(1R)-1-(naphthalen-2-yl)ethane-1,2-diol | C12 H12 O2 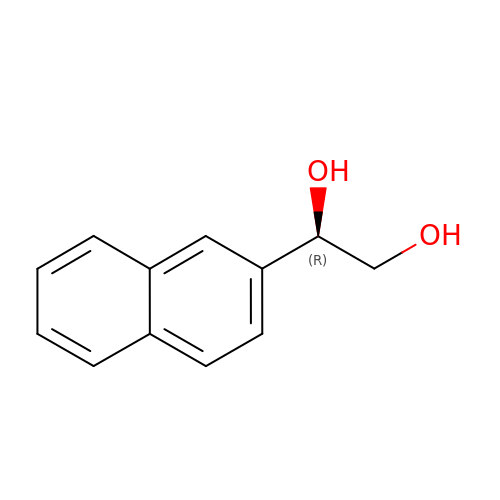| QFNOPZNUHSDHKZ-LBPRGKRZSA-N10-DECARBOXYMETHYLACLACINOMYCIN 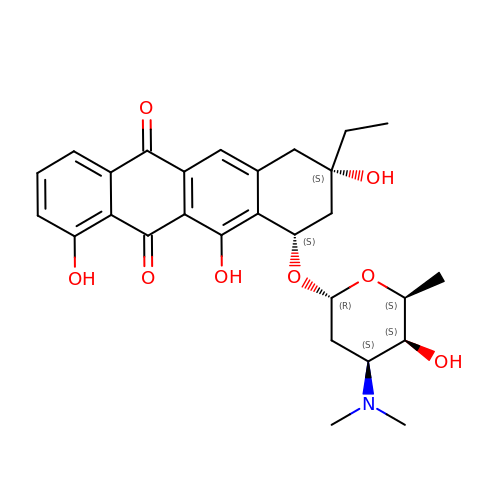T (DCMAT) | C28 H33 N O8 | BLGDWFJQIHBUJY-NWJGULHDSA-N(2S)-2-{[2-acetamido-2-deoxy-alpha-D-glucopyranosyl]oxy}butanedioic acid | C12 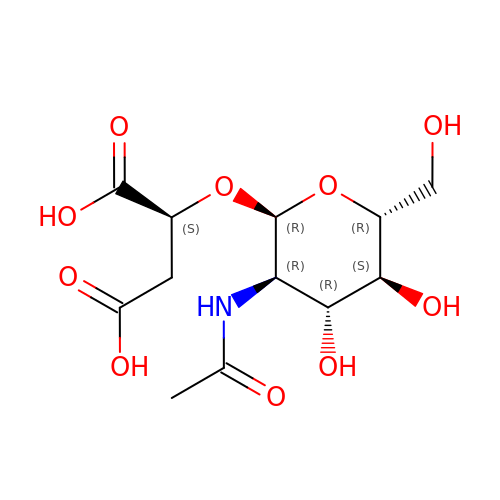H19 N O10 | COBMRTSHZAUOCY-BVKYVCSXSA-N(2R,3R,4R,5R,6R)-5-acetamido-2,3-difluoro-4-hydroxy-6-[(1R,2R)-1,2,3-trihydroxypropyl]tetrahydro-2H-pyran-2-carboxylic 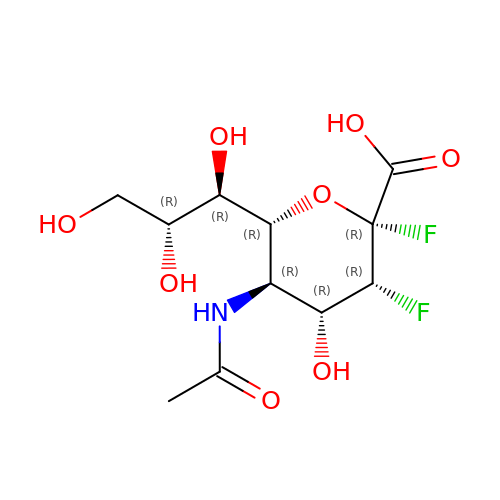acid | C11 H17 F2 N O8 | HMALKZAXODOYOP-DAXAGCIGSA-N> MTTLTLSEAAPLLKKEFREGRLIPFLGAGFSKPLKLPDGSQLIASLAKTLGFEPELFDMHGRFEQLAEFFAISAPNRLQRLVYEMSLSFDSAEAEALREKSPMHRALAALDWRTIYT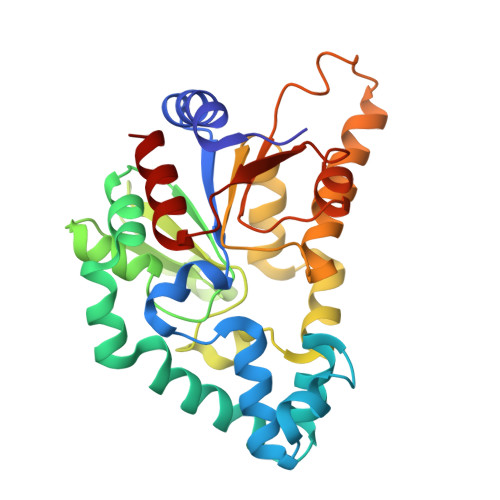TAYDKHVEGALRDAGKQAAVLASFADFQGPRARDVCEVIKFAGTLDQPDTIVLTESSYFQRMALDAPPDQRLRADLLANSFLFIGYSFSDTNIRYIWYRMNQLREQSQLGVKHSQARRCFFATHGAGLVQPDILQQWNIDVIQLDPTDKSASVARLLESIA> LSECKTGNGKNYRGTMSKTKNGITCQKWSSTSPHRPRFSPATHPSEGLEENYCRNPDNDPQGPWCYTTDPEKRYDYCDILECEEECMHCSGENYDGKISKTMSGLECQAWDSQSPH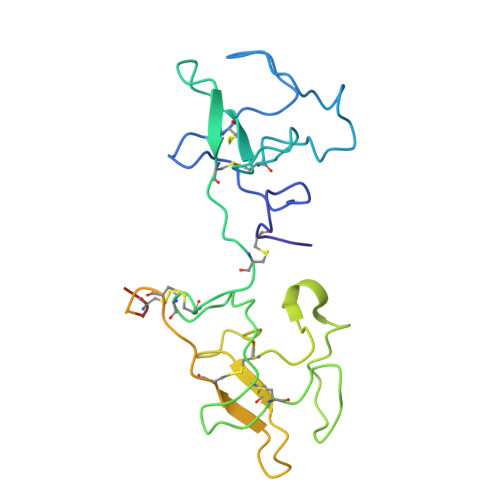AHGYIPSKFPNKNLKKNYCRNPDRELRPWCFTTDPNKRWELCDIPRCTTPPPSSGPTYQCLKGTGENYRGNVAVTVSGHTCQHWSAQTPHTHERTPENFPCKNLDENYCRNPDGKRAP>PMFIVNTNVPRASVPDGFLSE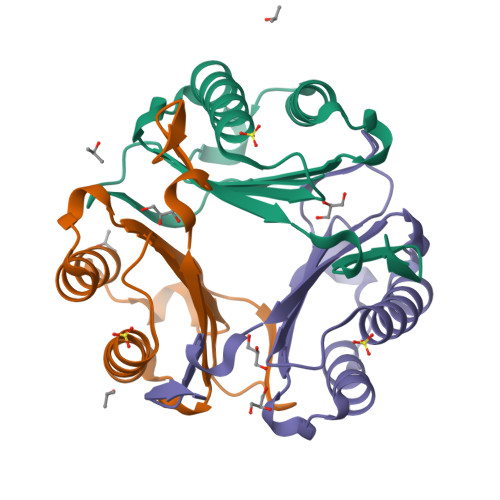LTQQLAQATGKPPQYIAVHVVPDQLMAFGGSSEPCALCSLHSIGKIGGAQNRSYSKLLCGLLAERLRISPDRVYINYFDMNAANVGWNNSTFA[3x]> GPLGSRIKTLSVSRPIIYGNTAKKMGSVKPPNAPAEHTHLWTIFVRGPQNEDISYFIKKVVFKLHDTYPNPVRSIEAPPFELTETGWGEFDINIKVYFVEEANEKVLNFYH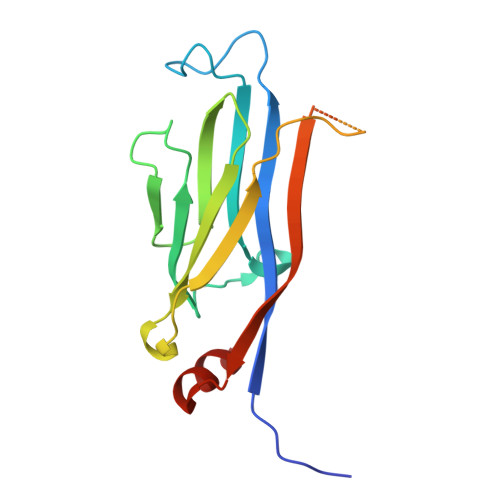RLRLHPYANPVPNSDNGNEQNTTDHNSKDAEVSSVYFDEIVFNEPNEEFFKILMSRPG> GSHMDINNKARIHWACRRGMRELDISIMPFFEHEYDSLSDDEKRIFIRLLECDDPDLFNWLMNHG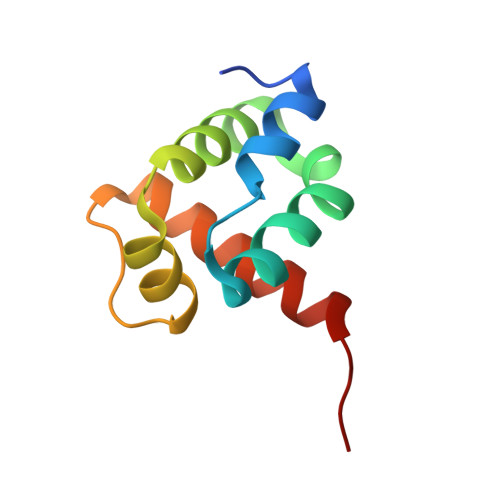KPADAELEMMVRLIQTRNRERGPVAI> MSTVHEILCKLSLEGDHSTPPSAYGSVKAYTNFDAERDALNIETAIKTKGVDEVTIVNILTNRSNAQRQDIAFAYQRRTKKELASALKSALSGHLETVILGLLKTPAQYDASELKASMKGLGTDEDSLIEIICSRTNQELQEINRVYKEMYKTDLEKDIISDTSGDFRKLMVALAKGRRAEDGSVIDYELIDQDARDLYDAGVKRKG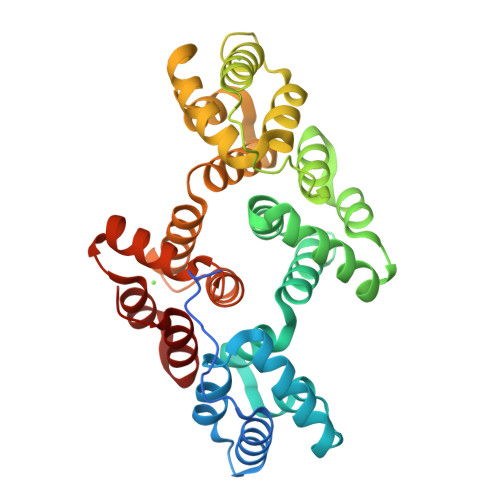TDVPKWISIMTERSVPHLQKVFDRYKSYSPYDMLESIRKEVKGDLENAFLNLVQCIQNKPLYFADRLYDSMKGKGTRDKVLIRIMVSRSEVDMLKIRSEFKRKYGKSLYYYIQQDTKGDYQKALLYLCGGDD TRI-CHLORO-ACETALDEHYDE | C2 H Cl3 O | 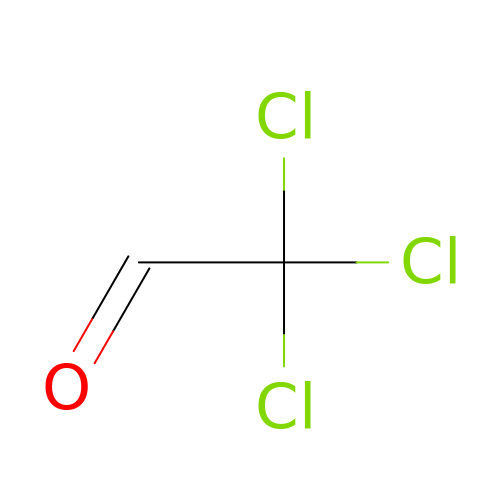HFFLGKNGCAIQMO-UHFFFAOYSA-N>SVDLIGINVAGAEFTGGKLPGKHGTHYFFPPEGYFEYWSEQGIHTVRFPLKWERLQPSLNAELDDVYASLVDDMLDQAKENDIKVILDVHNYARYRKKVIGTED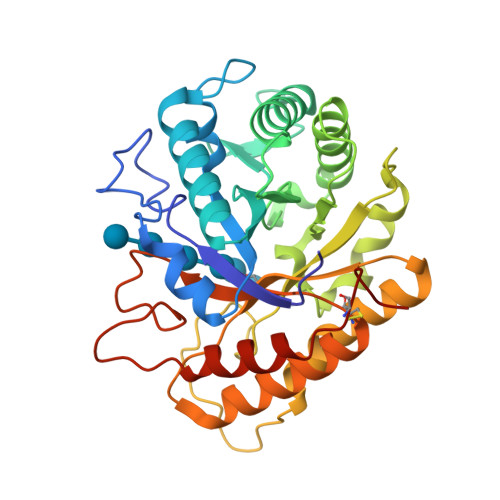VPVSAYQDLMERIAKRWQGHDALFAYDIMNEPYGSADKLWPAAAQAGIDGVRKYDKKRPLLIEGASWSSAARWPRYADELLKLKDPADNMVFSAHVFIDEDASGSYKKGPGKDFEPMIGVKRVEPFVNWLKEHGKKGHIGEFGIPNDDERWLDAMDKLLAYLNENCIPINYWAAGPSWGNYKLSIEPKDGEKRPQVALLKKYAAKDNCSDFGPAKAE[4x]> GASGSGTGSGSMSTLYLTQPDAVLSKKHEAFHVALKQEDGSWKKQPIPAQTLEDIVLLGYPSITGEALGYALELGLPVHYLTQFGKYVGSALPSESRNGQLRLAQFRAHEDPIQRLDIVKAFVKGKVHNQYNLLYRRGQVDNPLKGRGKLVMRQQTLEQVRGIEGLAAREYFASWQEMLGHEWTFTGRFRRPPTDPVNALLSFGYGLLRTQVTAAVHIAGLDPYIGFLHETTRGQPAMILDLMEEFRALVADSVVLTVLKQREIQRQDFTESLGAFRLTDSATKTFLGAFDRKLSSEFKHPIFNYKC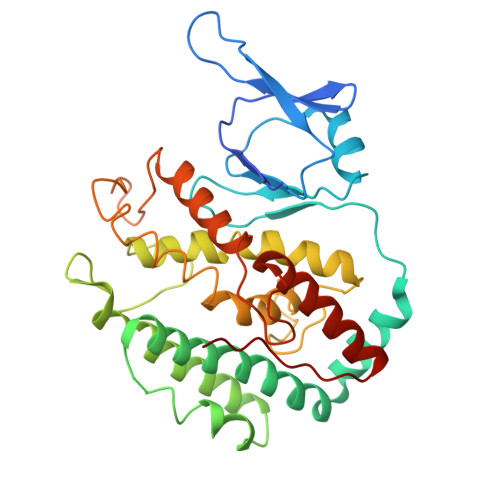TYRRAIELQARLLARHLQEGVVYEPLVIR Amplification of piRNA in the ping-pong cycle requires assembly of a tertiary complex scaffolded by Krimper, which simultaneously binds the N-terminal regions of Aub and Ago3. To promote generation of new piRNA, Krimper uses its two Tudor domains to bind Aub and Ago3 in opposite modification and piRNA-loading states. In addition to its self-interacting N-terminal region, Krimper contains two extended Tudor domains: eTud1(272-512) and eTud2 (562-746). Overall, our results reveal that the two Tudor domains of Krimper have distinct architectures that are responsible for the differential binding of two PIWI proteins.

To gain a detailed understanding of the interaction between Krimper (eTud2) and Aub, we undertook structural studies. We solved the crystal structure of the Krimper (eTud2) domain in complex with the Aub-R15me2 peptide that showed the highest binding affinity in ITC experiments. In the 2.7 Å structure the eTud2 domain adopted a typical Tudor subdomain and a staphylococcal nuclease (SN)-like subdomain (Tudor-SN) architecture. sDMA-modified Arg-containing peptide binds within a negatively-charged cleft between the Tudor and SN domains, and is specifically recognized by a conserved aromatic cage consisting of four aromatic amino acids Tyr624, Tyr630, Tyr646, and Tyr649, stabilized further by hydrophobic and cation-π interactions. In addition, eTud2 Asn651, which is conserved amongst other extended Tudor domains, forms a hydrogen bond with the guanidyl nitrogen of the methylated Arg15. Besides Arg15, other flanking arginine residues in the (G/A)R motif of Aub also contribute to protein-peptide binding. The binding pocket of eTud2 is similar to that of other Tudor domains and contains four aromatic residues that interact with sDMA. As sDMA modification of Aub signals its piRNA-binding status, the binding of eTud2 to modified Aub ensures that the complex contains Aub/piRNA.

>[8x]STTVHFEIGSIVGILITFINGPTEVYGQFLDGSPPLVWDKKDVPENKRTFKSKPRLLDIVLALYSDGCFYRAQIIDEFPSEYMIFYVDYGNTEFVPLSCLAPCENVDSFKPHRVFSFHIEGIVRSKNLTHQKTIECIEYLKSKLLNTEMNVHLVQRLPDGFLIRFLDDWKYIPEQLLQRNYAQVSQ;>[8x]NPVIARGRGRGRK> HHHHHHGLIQERRSHEVNPAAHLTGANSSLTGSGGPLLWETQLGLAFLRGLSYHDGALVVTKAGYYYIYSKVQLGGVGCPLGLASTITHGLYKRTPRYPEELELLVSQQS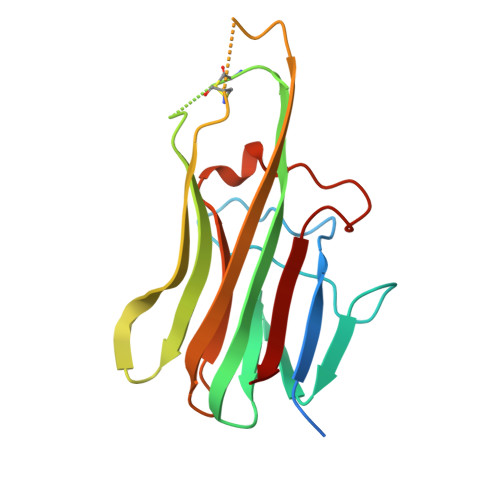PCGRATSSSRVWWDSSFLGGVVHLEAGEEVVVRVLDERLVRLRDGTRSYFGAFMV>GSHMANDSPAKSLVDIDLSSLRDPAGIFELVEVVGNGTYGQVYKGRHVKTGQLAAIKVMDVTEDEEEEIKLEINMLKKYSHHRNIATYYGAFIKKSPPGHDDQLWLVMEFCGAGSITDLVKNTKGNTLKEDWIAYISREILRGLAHLHIHHVIHRDIKGQNVLLTENAEVKLVDFGVSAQLDRTVGRRNTFIGTPYWMAPEVIACDENPDATYDYRSDLWSCGITAIEMAEGAPPLCDMHPMRALFLIPRNPPPRLKSKKWSKKFFSFIEGCLVKNYMQRPSTEQLLKHPFIRDQPNERQ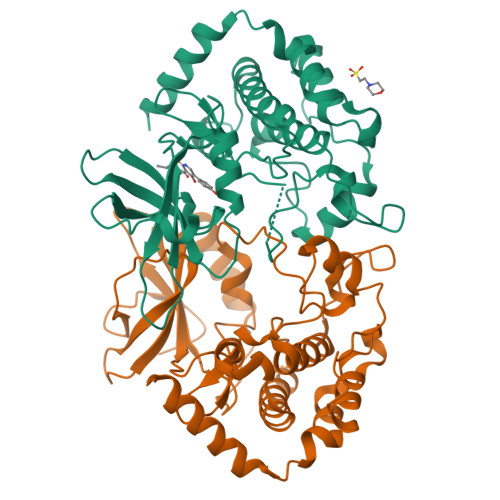VRIQLKDHIDRTRKKRGEKDETEYEYSG[2x]>MPRVKAAQAGRQSSAKRHLAEQFAVGEIITDMAAAAWKVGLPIGQGGFGCIYLADMNSSESVGSDAP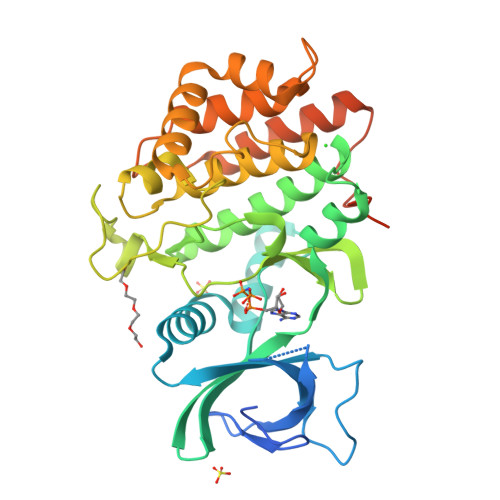CVVKVEPSDNGPLFTELKFYQRAAKPEQIQKWIRTRKLKYLGVPKYWGSGLHDKNGKSYRFMIMDRFGSDLQKIYEANAKRFSRKTVLQLSLRILDILEYIHEHEYVHGDIKASNLLLNYKNPDQVYLVDYGLAYRYCPEGVHKAYAADPKRCHDGTIEFTSIDAHNGVAPSRRGDLEILGYCMIQWLTGHLPWEDNLKDPKYVRDSKIRYRENIASLMDKCFPAANAPGEIAKYMETVKLLDYTEKPLYENLRDILLQGLKAIGSKDDGKLDLSVVENGGLKAKTITKKRAAEIEEHHHHHH[4x]> GPQRNGRAPEGKMDLIIMRGDKGFGFRLSGATHSAAEQTAQGQWVRNVD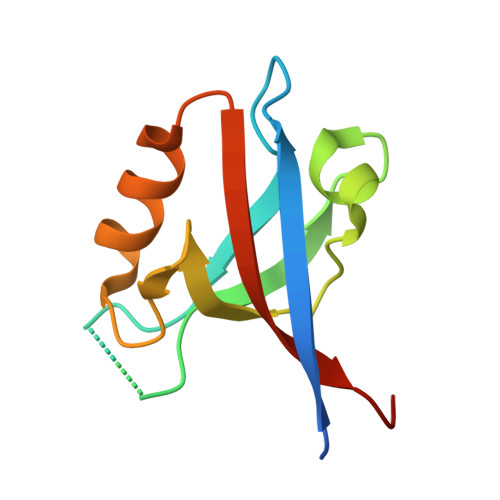PDGQAARAGLQAGDRLLELNGVDVSFWSHRKVVDEIKRSGDVVAFRIARRLSPGPD> MIGIDIVSIARIEKCVKRFKMKFLERFLSPSEIVLCKDKSSSIAGFFALKEACSKALQVGIGKELSFLDIKISKSPKNAPLITLSKEKMDYFNIQSL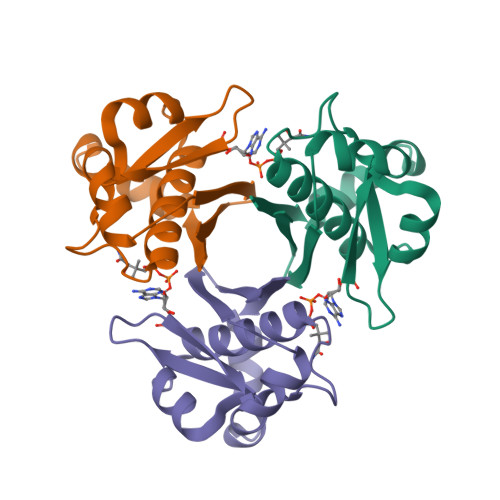SASISHDAGFAIAVVVVSSSNE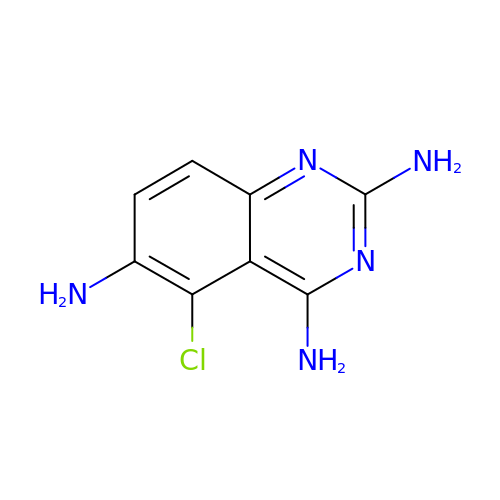5-CHLORYL-2,4,6-QUINAZOLINETRIAMINE | C8 H8 Cl N5 | JZWXVYNQIJJTKF-UHFFFAOYSA-N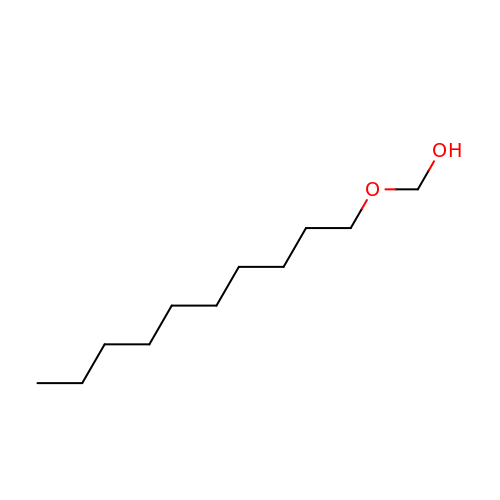DECYLOXY-METHANOL | C11 H24 O2 | CDMVCFBAVCCGIE-UHFFFAOYSA-N2-(2-HYDROXY-CYCLOPENTYL)-PENT-4-ENAL 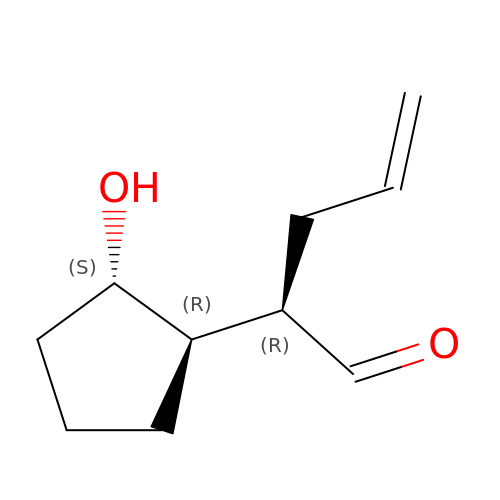| C10 H16 O2 | NEWBFDLFXDTFGD-AEJSXWLSSA-N>[2x]PTMEGPLRRKTLLKEGRKPALSSWTR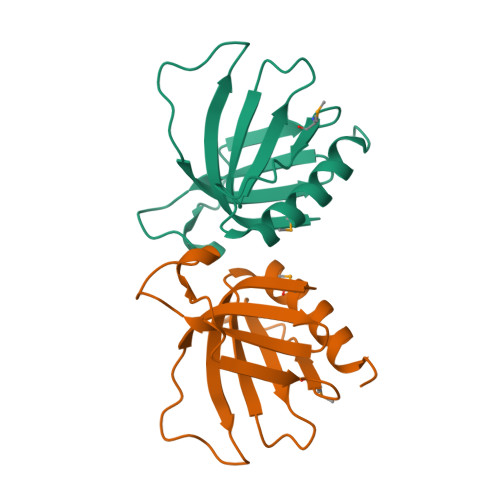YWVVLSGATLLYYGAKSLRGTDRKHYKSTPGKKVSIVGWMVQLPDDPEHPDIFQLNNPDKGNVYKFQTGSRFHAILWHKHLDDACKSSRPQVPANLMSFE> SSEPCCDSCRCTKSIPPQCHCANI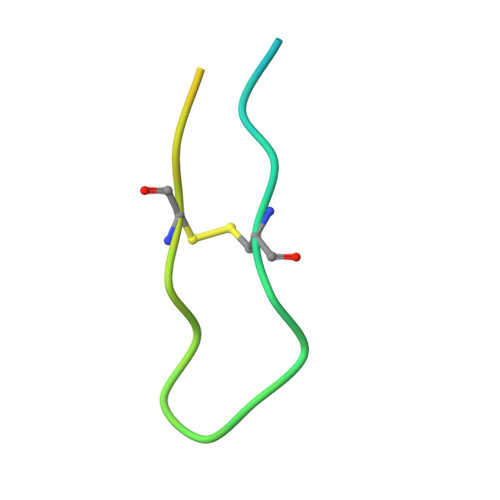RLFCYKPCESM> MVRGIRGAITVEEDTPAAILAATIELLLKMLEANGIQSYEELAAVIFTVTEDLTSAFPAEAARLIGMHRVPLLSAREVPVPGSLPRVIRVLALWNTDTPQDRVRHVYLNEAVRLRPDLES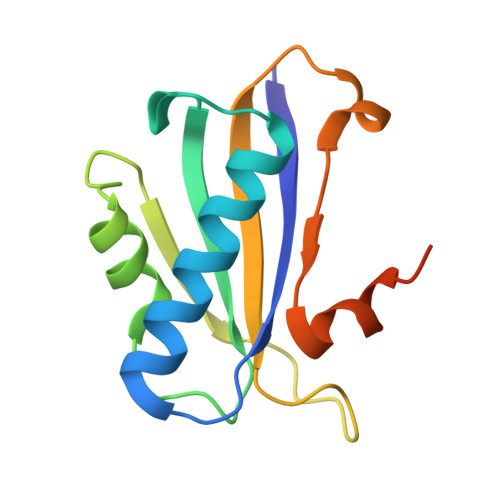AQLEHHHHHH>MGLNFFRKAAPEVRTEPVAERKASVTGRIVAMASGAGRPVWGPRDTVSLMRTGFAGNPVGFRSVKLIAEATAAVPLICQDAERRYEIHPVLDLLRRPNAGQGRAELFEALIGQILLSGNGYLEAVCPEPGVPRELHVLRSDRMAVVPGADGWPVGYDYTVGGRKHRFDMTGHPDPICHIKSFHPTDDHYGLSPMQAAAVALDVHNAASAWSKALLDNAARPSGAIIYKGADGQGVLAPEQYERLIFEMETHHQGARNAGRPMLLEGGLDWKPMGFSPSDMEFHETKAAAAREIALAFGVPPMLIGIPGDATYANYAEANRAFYRLTVLPLLTRVSAALAWWLSGYLGAQIELKPDLDQVPALAVERDQLWARIGAAGFLSNSEKRVLLGLPPTAEG[2x];>MMLNEVTAVPGTALPVAEFRDHLRLGTGFADLGAEDAALLSYLRAAIAAIEGRTAKALISRGFRLALTAWRWGDMQTLPIAPVATVTALRLVDAAGVETPVAAGWRLVPDMARPRIEALGAMLPMIPTGGRVEIDFTAGFGASWSALPVDLAQAVFLLAAQYYELRHDGAAEGGAMPFGVMALIERWRTVRVLGGRP[2x];> MSRPRLNRLLVLEEAVRVADGAGGHRLDWQAKGEVWAEVTAGSGSERAGEFVTLASVPFTIVVRAAPVGAARRPRPEQRFREGARIFRILAVAERDREGHYLSCFAREEVVA;> MSYAVAGALQAAVYQQLRADAVLAALVGTAVYDAVPPGPLAGTYVSLGPEDVADASDKTGAGAVHDFVISVITDAAGFATAKAAAAAVSDALVGADLVLSRGRLVGLWFLRAKARRVEKADMRRIDLVFRARVE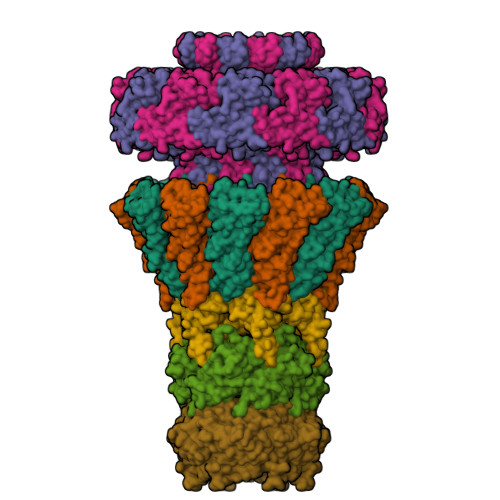G;> MAAQNGKDLLIKLDLTGSGQFETIAGLRATRISFNAETVDVTSLESQGGWRELLGGAGVRSASISGAGVFKDADTDERARQIFFDGEVPEFQVIIPDFGIVQGPFMITSIDYAGSHNGEASYELAMASAGALSFTAI>[4x]MTSASSPPAFRLETSDGDEEGNAEVNKGKQEPPPMESPFQREDRNSSPQIKVNLNFIKRPPKNTSAPSQQEPDRFDRDRLFSVVSRGVPEELTGLLEYLRWNSKYLTDSAYTEGSTGKTCLMKAVLNLQDGVNACIMPLLQIDKDSGNPKLLVNAQCTDEFYQGHSALHIAIEKRSLQCVKLLVENGADVHLRACGRFFQKHQGTCFYFGELPLSLAACTKQWDVVTYLLENPHQPASLEATDSLGNTVLHALVMIADNSPENSALVIHMYDGLLQMGARLCPTVQLEEISNHQGLTPLKLAAKEGKIEIFRHILQREFSGPYQPLSRKFTEWCYGPVRVSLYDLSSVDSWEKNSVLEIIAFHCKSPNRHRMVVLEPLNKLLQEKWDRLVSRFFFNFACYLVYMFIFTVVAYHQPSLDQPAIPSSKATFGESMLLLGHILILLGGIYLLLGQLWYFWRRRLFIWISFMDSYFEILFLLQALLTVLSQVLRFMETEWYLPLLVLSLVLGWLNLLYYTRGFQHTGIYSVMIQKVILRDLLRFLLVYLVFLFGFAVALVSLSREARSPKAPEDNNSTVTEQPTVGQEEEPAPYRSILDASLELFKFTIGMGELAFQEQLRFRGVVLLLLLAYVLLTYVLLLNMLIALMSETVNHVADNSWSIWKLQKAISVLEMENGYWWCRRKKHREGRLLKVGTRGDGTPDERWCFRVEEVNWAAWEKTLPTLSEDPSGPGITGNKKNPTSKPGKNSASEEDHLPLQVLQSP

Transient receptor potential vanilloid (TRPV) channels are a group of six polymodal cation channels subdivided into two subgroups by their sequence identity and functional properties. TRPV1–TRPV4 comprise the first subgroup of non-selective Ca2+ channels, TRPV5 and TRPV6 constitute the second subgroup of Ca2+ selective channels. TRPV channels are blocked by ruthenium red (RR), a universal pore blocker for a wide array of cation channels. Here we use cryo-electron microscopy to reveal the molecular details of RR block in TRPV2 and TRPV5, members of the two TRPV subfamilies.

We also prepared cryo-EM grids of TRPV2 in the presence of 1 mM RR without the activator. The dataset yielded a single stable state with unique and strong density at the SF: RR-bound TRPV2 (TRPV2RR) in C1 at 3.3 Å resolution with a wide SF and closed lower gate (Figure EV2). The presence of RR stabilized the TRPV2RR SF in the TRPV2Apo2-like state but did not reveal the expected shape for the RR molecule (Figure EV2). The TRPV2RR SF harbors a large asymmetric density coordinated by Glu609 and the Gly606 backbone carbonyls from only some of the TRPV2 monomers (Figure EV2). TRPV2 has a flexible and adaptable SF which can easily allow for the entrance of the bulky RR while the channel is in the TRPV2Apo2 conformation with the open SF. Yet RR is not tightly coordinated in this position, resulting in somewhat amorphous density. Thus, our results agree with the previous observation that the TRPV1-TRPV3 SF is dynamic and can permit cation passage even when the pore is closed at the lower gate.N-[(2R)-2-{[3-(3'-chlorobiphenyl-4-yl)-1,2-oxazol-5-yl]methyl}-4-(hydroxyamino)-4-oxobutanoyl]-L-alpha-glutamyl-L-alpha-glutamine | C30 H32 Cl N5 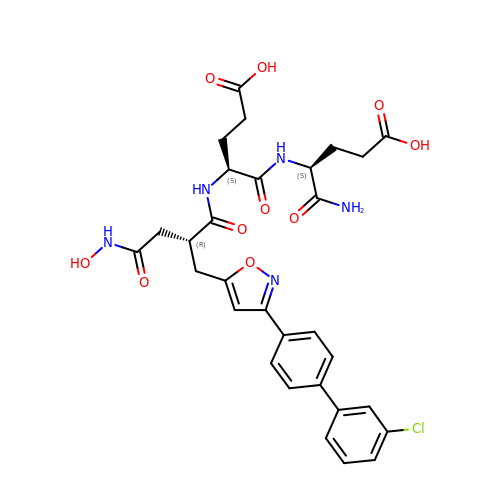O10 | VBMQORMYXJZHKU-OIBXWCBGSA-N> MSVEDTQPLITHLIELRKRLLNCIIAVIVIFLCLVYFANDIYHLVSAPLIKQLPQGSTMIATDVASPFFTPIKLTFMVSLILSAPVILYQVWAFIAPALYKHERRLVVPLLVSSSLLFYIGMAFAYFVVFPLAFGFLANTAPEGVQVSTDIASYLSFVMALFMAFGVSFEVPVAIVLLCWMGITSPEDLRKKRPYVLVGAFVVGMLLTPPDVFSQT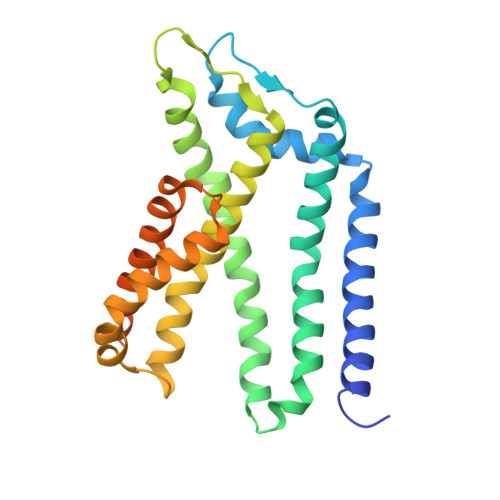LLAIPMYCLFEIGVFFSRFYVGKGRNREEENDAEAESEKTEERSHHHHHH> SPNGQTKPLPALKLALEYIVPCMNKHGICVVDDFLGKETGQQIGDEVRALHDTGKFTDGQLVSQKSDSSKDIRGDKITWIEGKEPGCETIGLLMSSMDDLIRHCNGKLGSYKINGRTKAMVACYPGNGTGYVRHVDNPNGDGRCVTCIYYLNKDWDAKVSGGILRIFPEGKA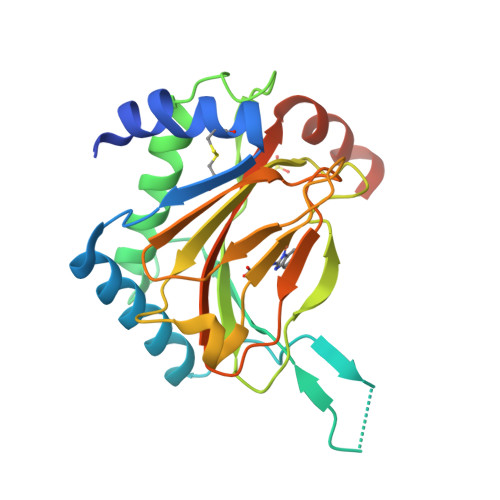QFADIEPKFDRLLFFWSDRRNPHEVQPAYATRYAITVWYFDADERARAKVKYLTGEKGVRVELNK>[2x]ALVIAFIGKNGAVMAGDMREITFEGEKPDREKLEKELYSGSIVTDEEMQKKAEEFGVKITVADCKEKVSERNGVLVGEVSSAEGGVVKKRRLYASAGNFAIAELINTEMTLTSQGKGSNFIAFGNEFTKQVANKCFKDNWTKKSNLQDAVKILILCMETVARKTASVSKQFMIVQTASNADVLKVVEKDRNC

The discovery of peptide ligase activity in the Connectase family of enzymes (CETs) from archaea has expanded protease repurposing strategies. However, original CETs exhibit significant residual protease activity, leading to nonprocessive (reversible) ligation and limiting their application. In this study, we present crystal structures of a highly active protein ligase from Methanococcus maripaludis (MmCET) in both its apo- and substrate-bound forms. By determining the crystal structure of MmCET, both with and without a preferred peptide substrate at its catalytic transition state, we uncovered the essential elements responsible for the high-precision substrate recognition of N-terminal motifs.

To this end, we first attempted to capture MmCET in both its apo form and its peptide substrate-bound form. In this conformation, cysteines in MmCET form a stable intermolecular disulfide bond (C65–C193), locking the enzyme in a dimeric state and constraining the crystal lattice. Interestingly, removing these cysteines via site-directed mutagenesis did not affect the crystallization, and ligand-free enzymes were still observed in the same crystal form. Moreover, volume analysis of the substrate pocket of the free MmCET structure revealed significant potential for designing more favorable peptide substrates.>HHHHHHGSKWTSTAIITQPDVGQIAGYNNAMNVIYGQAAPKVSDLQETLIGRFSSAFSALAETLDNQEEPEKLTIEPSVKNQQLPLTVSYVGQTAEGAQMKLAQYIQQVDDKVNQELEKDLKDNIALGRKNLQDSLRTQEVVAQEQKDLRIRQIQEALQYANQAQVTKPQVQQTEDVT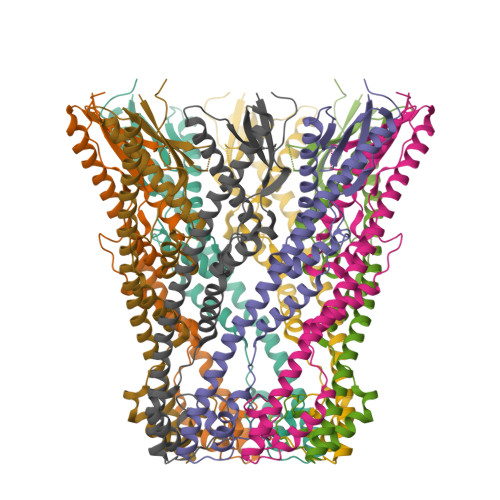QDTLFLLGSEALESMIKHEATRPLVFSPNYYQTKQTLLDIKNLKVTADTVHVYRYVMKPTLPVRRDS[2x]> MQTLHALLRDIPAPDAEAMARTQQHIDGLLKPPGSLGRLETLAVQL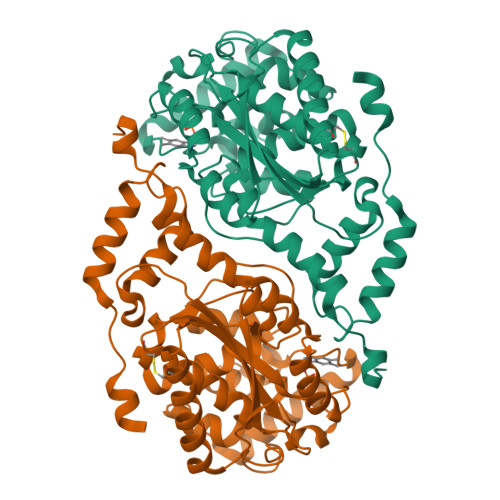AGMPGLNGTPQVGEKAVLVMCADHGVWDEGVAVSPKIVTAIQAANMTRGTTGVCVLAAQAGAKVHVIDVGIDAEPIPGVVNMRVARGCGNIAVGPAMSRLQAEALLLEVSRYACDLAQRGVTLFGVGELGMANTTPAAAMVSVFTGSDAKEVVGIGANLPPSRIDNKVDVVRRAIAINQPNPRDGIDVLSKVGGFDLVGMTGVMLGAARCGLPVLLDGFLSYSAALAACQIAPAVRPYLIPSHFSAEKGARIALAHLSMEPYLHMAMRLGEGSGAALAMPIVEAACAMFHNMGELAASNIVLPEGNANAT> HHHHHHGSNRTVTVEELPIDPANVAAYAAVTGLRYGNQVPLTYPFALTFPSVMSLVTGFDFPFAAMGAIHTENHITQYRPIAVTDAVGVRVRAENLREHRRGLLVDLVTNVSVGNDVAWHQVTTFLHQQRTSLSGEPKPPPQKKPKLPPPAAVLRITPAKIRRYAAVGGDHNPIHTNPIAAKLF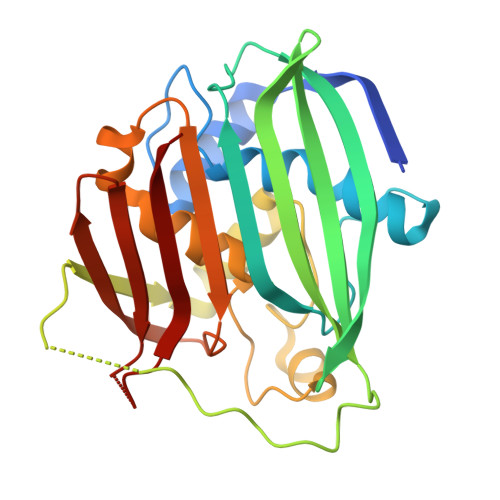GFPTVIAHGMFTAAAVLANIEARFPDAVRYSVRFAKPVLLPATAGLYVAEGDGGWDLTLRNMAKGYPHLTATVRGL FabZ is an important enzyme responsible for elongation cycle of both saturated and unsaturated fatty acid biosynthesis in FAS II pathway that is essential for membrane formation in bacteria, and it has been recognized as an attractive target for antibacterial drug discovery. Six monomers of the hexamer arranged a ring-like contact topology (A-B-F-E-C-D-A), and every two monomers (A/B, C/D and E/F) formed dimer each other through hydrophobic interactions. Two L-shaped substrate-binding tunnels with the entrance protected by a door residue Tyr100 were located in the interface of a dimer and ~20 Å away from each other. The catalytic site in the tunnel was formed by two highly conserved residues, His58 and Glu72' that were located in the middle kink of the tunnel.

Emodin was discovered as the inhibitor of HpFabZ by IC50 value of 9.7 ± 1.0 μM and further inhibition mode characterization suggested that it functioned as a competitive HpFabZ inhibitor with Ki value of 1.9 ± 0.3 μM. Emodin inhibited HpFabZ activity by either binding to Tyr100 or embedding into the middle of the tunnel C appropriately with favorable shape of complementary, thus preventing the substrate from accessing the active site. Different from the open and close conformations, the phenol ring of door residue Tyr100 flopped ~120° to a third conformation and paralleled the pyrrolidine ring of Pro112'. Ring A of Emodin was then stacked between the phenol ring and pyrrolidine ring forming a sandwich structure, while 3'-methyl of ring A also interacted with residues Arg110 and Ile111 via hydrophobic interactions. Apart from the interactions between ring A and residues near the tunnel entrance, ring C of Emodin also formed Vander Waals interactions with residues Phe59' and Ile98, and was stabilized in the right place by the hydrogen bond interaction between 6'-hydroxyl of ring C and water molecule 466 which formed H-bond to Oε2 of Glu159. In the other binding model (designated hereinafter as model B in Fig. 4C), Emodin entered into the middle of the tunnel C near the catalytic site, and located in the hydrophobic pocket consisting of residues Ile20, Leu21, Pro22, His23, Gly79, Phe83, Ile98, Val99 and Phe101. Ring A extended to the bottom of the tunnel and was stacked between residues Pro22 and Ile98, ring B interacted with residue Val99, while ring C bound to residues His23 and Phe101 through hydrophobic interactions. Additional hydrophobic interactions between 3'-methyl of ring A and residues Ile20 and Phe83, and hydrogen bond interactions between 6'-hydroxyl of ring C and water molecules of W12 and W402 which formed H-bonds to Oε1 and Oε2 of Glu72 respectively stabilized Emodin in the right place. The structural analysis indicated that the inhibitors specifically bound to tunnels B and C rather than the other four active tunnels of HpFabZ hexamer.

>MEQSHQNLQSQFFIEHILQILPHRYPMLLVDRITELQANQKIVAYKNITFNEDVFNGHFPNKPIFPGVLIVEGMAQSGGFLAFTSLWGFDPEIAKTKIVYFMTIDKVKFRIPVTPGDRLEYHLEVLKHKGMIWQVGGTAQVDGKVVAEAELKAMIAERE[6x]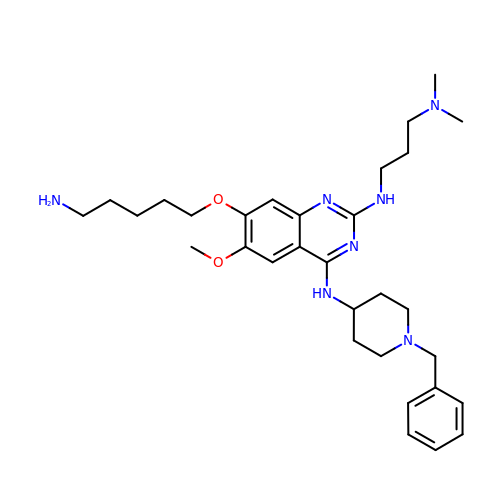7-[(5-aminopentyl)oxy]-N~4~-(1-benzylpiperidin-4-yl)-N~2~-[3-(dimethylamino)propyl]-6-methoxyquinazoline-2,4-diamine | C31 H47 N7 O2 | KJNBMUDJPFXUTG-UHFFFAOYSA-N>SNASVIVGRALPEVRDGLKPVHRRVLYAMFDSGFRPDRSHAKSARSVAETMGNYHPHGDASIYDSLVRMAQPWSLRYPLVDGQGNFGSPGNDPPAAMRYTEARLTPLAMEMLREIDEETVDFIPNYDGRVQEPTVLPSRFPNLLANGSGGIAVGMATNIPPHNLRELADAVFWALENHDADEEETLAAVMGRVKGPDFPTAGLIVGSQGTADAYKTGRGSIRMRGVVEVEEDSRGRTSLVITELPYQVNHDNFITSIAEQVRDGKLAGISNIEDQSSDRVGLRIVIEIKRDAVAKVVINNLYKHTQLQTSFGANMLAIVDGVPRTLRLDQLIRYYVDHQLDVIVRRTTYRLRKANERAHILRGLVKALDALDEVIALIRASETVDIA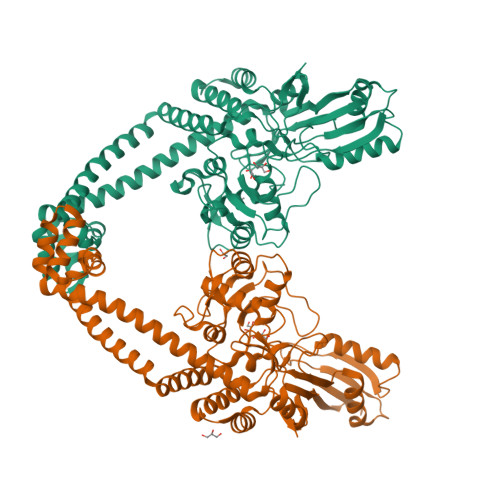RAGLIELLDIDEIQAQAILDMQLRRLAALERQRIIDDLAKIEAEIADLEDILAKPERQRGIVRDELAEIVDRHGDDRRTRIIA[2x]>GAKSEMAFAGKGEISPRAITMWDFSWLERRWPGAGYEDW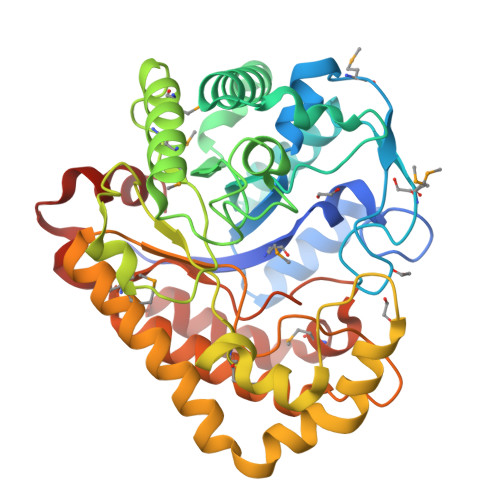DQVLDELSERGYNAIRIDAYPHLIAENPMKKWLLKEVWNQQDWGSPDMNEVQVQPNLNLFLSKCKERDIKVGLSSWYRLDVDEVCLKLDTPEKLADCWLTILRSIEEDGLLDTILYVDLCNEWPGDSWAPFFAKTYPNVGWGNWYKEESLRWMKTSLEKMRQVYPDMPFLYSFDHGDVKKYEEVDCSFLDLYEHHIWMAQQNGGEFYKLVGYGYNRFLPDDYKNVVKNAERVYRERPGYWQKLLTDKIELMASVARKNRRPLVTTECWGLVDYKDWPLLKWDWVKDLCELGTITAARTGMWVGVATSNFCGPQFAGMWRDVEWHKRLTSIIRSSPLDESLTKNNEVAAKLLKRL[2x]>GHMDLKTAVFNAARDGKLRLLTKLLASKSKEEVSSLISEKTNGATPLLMAARYGHLDMVEFLLEQCSASIEVGGSVNFDGETIEGAPPLWAASAAGHLKVVQSLLNHGASVNNTTLTNSTPLRAACFDGHLEIVKYLVEHKADLEVSNRHGHTCLMISCYKGHKEIAQYLLEKGADVNRKSVKGNTALHDCAESGSLDIMKMLLMYCAKMEKDGYGMTPLLSASVTGHTNIVDFLTHHAQTSKTERINALELLGATFVDKKRDLLGALKYWKKAMNMRYSDRTNIISKPVPQTLIMAYDYAKEVNSAEELEGLIADPDEMRMQALLIRERILGPSHPDTSYYIRYRGAVYADSGNFKRCINLWKYALDMQQSNLDPLSPMTASSLLSFAELFGGGSGGGS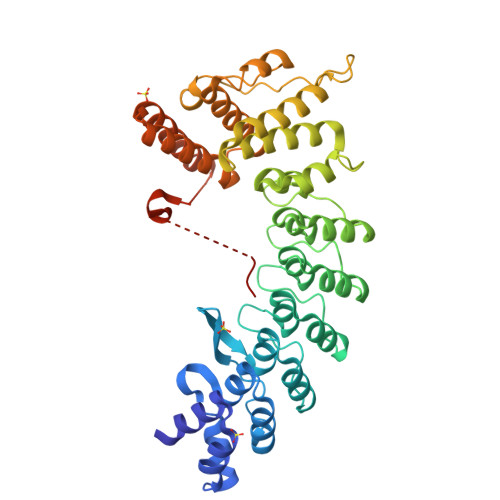GGGSGGGSRLLSKHRFSR[2x]4-(2-chlorophenyl)-8-[3-(dimethylamino)propoxy]-9-hydroxy-6-methylpyrrolo[3,4-c]carbazole-1,3(2H,6H)-dione 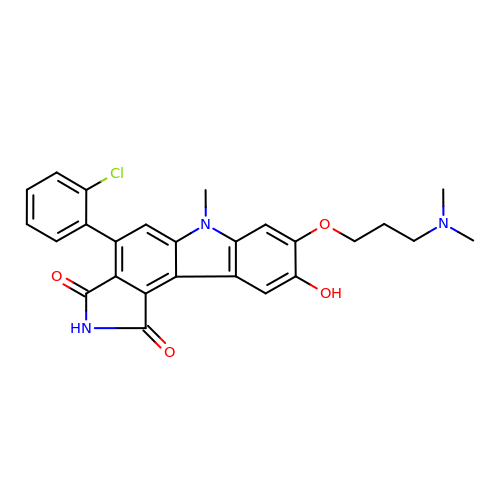| C26 H24 Cl N3 O4 | ZWRDUCSPTGMSHB-UHFFFAOYSA-N> GAMSGGLLKALRSDSYVELSQYRDQHFRGDNEEQEKLLKKSCTLYVGNLSFYTTEEQIYELFSKSGDIKKIIMGLDKMKKTACGFCFVEYYSRADAENAMRYINGTRLDDRIIRTDWDAGFKEGRQYGRGRSGGQVR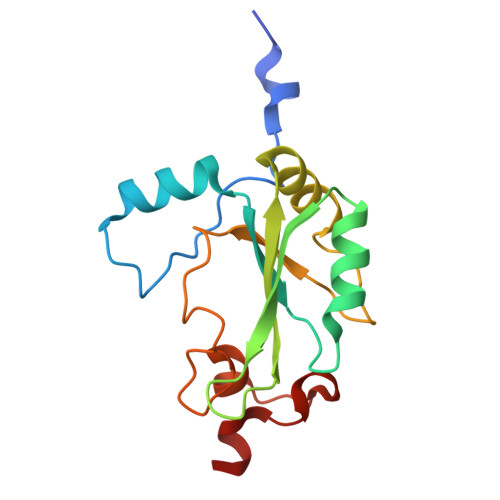DEYRQDYDAGRGGYGKLAQNQ> MFEARLVQGSILKKVLEALKDLINEACWDISSSGVNLQSMDSSHVS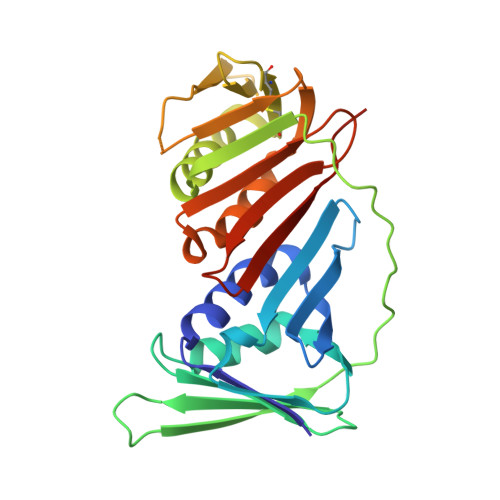LVQLTLRSEGFDTYRCDRNLAMGVNLTSMSKILKCAGNEDIITLRAEDNADTLALVFEAPNQEKVSDYEMKLMDLDVEQLGIPEQEYSCVVKMPSGEFARICRDLSHIGDAVVISCAKDGVKFSASGELGNGNIKLSQTSNVDKEEEAVTIEMNEPVQLTFALRYLNFFTKATPLSSTVTLIMSADVPLVVEYKIADMGHLKYYLAPKIEDEEGS>[4x]MDYKDDDDKGRLRRRQEIIDHEEEESNDDVSSRRGKLSLAETFRWLDSSEHRRIETDGHNDYKYIIHPKNRWYKAWEMFILVWAIYSSLFTPMEFGFFRGLPERLFVLDIVGQIAFLVDIVLQFFVAYRDTQTYRTVYKPTRIAFRYLKSHFLMDFIGCFPWDLIYKASGKHELVRYLLWIRLFRVRKVVEFFQRLEKDTRINYLFTRILK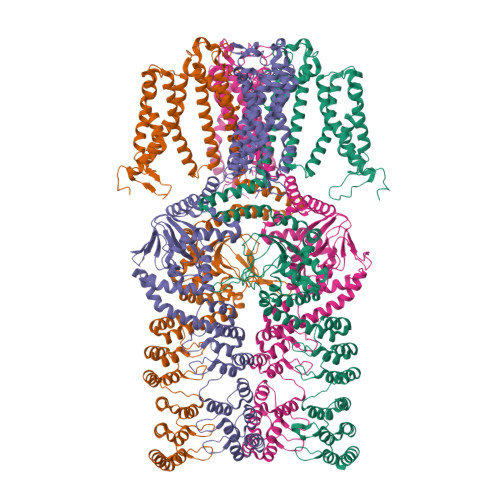LLFVEVYCTHTAACIFYYLATTLPPENEGYTWIGSLKLGDYSYENFREIDLWKRYTTALYFAIVTMATVGYGDIHAVNLREMIFVMIYVSFDMVLGAYLIGNITALIVKGSNTERFRDKMNDLISFMNRKKLGRDLRSQITGHVRLQYDSHYTDTVMLQDIPASIRAKIAQLLYLPYIKKVPLFKGCSTEFINQIVIRLHEEYFLPGEVITEQGNVVDHLYFVCEGLLEALVTKTDGSEESVTLLGPHTSFGDISIICNISQPFTVRVCELCHLLRLDKQSFSNILEIYFHDGRTILNNIMEEKESNDRIKKLESDIVIHIGKQEAELALKVNSAAFQGDFYQLKSLIRSGADPNKTDYDGRSPLHLAACRGYEDITLFLIQEGVDVNLKDKFGHTPLFEAVKAGQEGVIGLLVKEGASFNLEDSGNFLCTTVAKGDSDFLKRLLSSGMNPNSEDYDHRTPLHVAASEGLFLMAKMLVEAGASVISKDRWGNSPLDEARLCGNKKLIKLLEDVKNAQSSIYPSSLRELQEERIERRKCTVFPFHPQEAKEERSRKHGVVVWIPSNLEKLIVTAAKELGLSDGASFVLLSEDQGRITDIDMISDGHKLYMISDTTDQTHHHHHH>MFSIPPLPWGYDGLAAKGLSKQQVTLHYDKHHQGYVTKLNAAAQTNSALATKSIEEII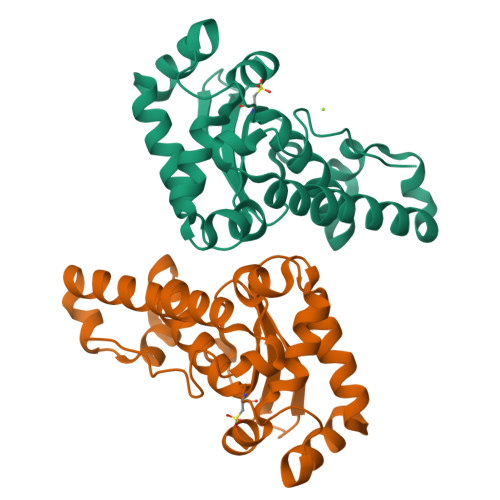RTEKGPIFNLAAQIFNHTFYWESMCPNGGGEPTGKVADEINASFGSFAKFKEEFTNVAVGHFGSGWAWLVKDTNSGKLKVYQTHDAGCPLTEPNLKPLLTCDVWEHAYYVDYKNDRAAYVQTFWNVVNWKNVERQL[2x]> MAAPNRDPPGYRYAAAMVPTGSLLSTIEVASHRRLFDFFSRVRSDANSLYDVEFDALLGSYCNTLSLVRFLELGLSVACVCTKFPELAYMNEGRVQFEVHQPLIARDGPHPIEQPTHNYMTKIIDRRALNAAFSLATEAIALLTGEALDGTGISAHRQLRAIQQLARNVQAVLGAFERGTADQMLHVLLEKAPPLALLLPMQRYLDNGRLATRVARATLVAELKRSFCETSFFLGKAGHRREAVEAWLVDLTTATQPSVAVPRLTHADTRGRPVDGVLVTTAPIKQRLLQSFLKVEDTEADVPVTYGEMVLNGANLVTALVMGKAVRSLDDVGRHLLEMQEEQLDLNRQTLDELESAPQTTRVRADLVSIGEKLIFLEALEKRIYAATNVPYPLVGAMDLTFVLPLGLFNPVMERFAAHAGDLVPAPGHPDPRAFPPRQLFFWGKDRQVLRLSLEHAIGTVCHPSLMNVDAAVGGLNRDPVEAANPYGAYVAAPAGPAADMQQLFLNAWGQRLAHGRVRWVAEGQMTPEQFMQPDNANLALELHPAFDFFVGVADVELPGGDVPPAGPGEIQATWRVVNGNLPLALCPAAFRDARGLELGVGRHAMAPATIAAVRGAFEDRNYPAVFYLLQAAIHGSEHVFCALARLVVQCITSYWNNTRCAAFVNDYSLVSYVVTYLGGDLPEECMAVYRDLVAHVEALAQLVDDFTLTGPELGGQAQAELNHLMRDPALLPPLVWDCDALMRRAALDRHRDCRVSAGGHDPVYAAACNVATADFNRNDGQLLHNTQARAADAADDRPHRGADWTVHHKIYYYVMVPAFSRGRCCTAGVRFDRVYATLQNMVVPEITPGEDCPSDPVTDPAHPLHPANLVANTVNAMFHNGRVVVDGPAMLTLQVLAHNMAERTTALLCSAAPDAGANTASTTNMRIFDGALHAGILLMAPQHLDHTIQNGDYFYPLPVHALFAGADHVANAPNFPPALRDLSRQVPLVPPALGANYFSSIRQPVVQHVRESAAGENALTYALMAGYFKISPVALHHQLKTGLHPGFGFTVVRQDRFVTENVLFSERASEAYFLGQLQVARHETGGGVNFTLTQPRGNVDLGVGYTAVVATATVRNPVTDMGNLPQNFYLGRGAPP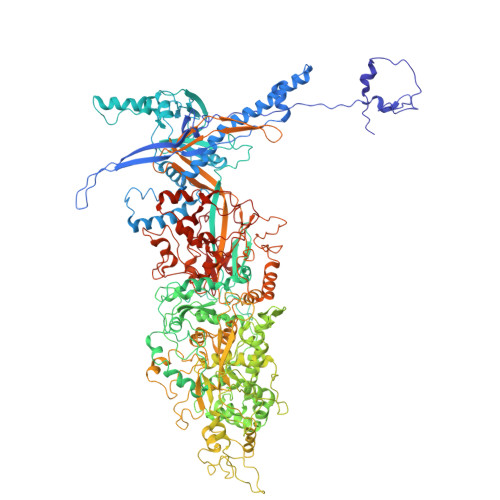LLDNAAAVYLRNAVVAGNRLGPAQPVPVFGCAQVPRRAGMDHGQDAVCEFIATPVSTDVNYFRRPCNPRGRAAGGVYAGDKEGDVTALMYDHGQSDPSRAFAATANPWASQRFSYGDLLYNGAYHLNGASPVLSPCFKFFTSADIAAKHRCLERLIVETGSAVSTATAASDVQFKRPPGCRELVEDPCGLFQEAYPLTCASDPALLRSARNGEAHARETHFAQYLVYDASPLKGLAL Defense-associated sirtuin 2 (DSR2) systems are widely distributed across prokaryotic genomes, providing robust protection against phage infection. DSR2 recognizes phage tail tube proteins and induces abortive infection by depleting intracellular NAD+, a process that is counteracted by another phage-encoded protein, DSR Anti Defense 1 (DSAD1). Each DSR2 protomer consists of a conserved N-terminal Sirtuin (SIR2) domain, a C-terminal domain (CTD) and a middle domain (MD). DSR2 assembles into an elongated tetramer, with four NADase catalytic modules clustered in the center and the regulatory-sensing modules distributed at four distal corners.

To understand the structural basis of DSR2 anti-phage defense, we expressed the full-length Bacillus subtilis DSR2 protein in Escherichia coli BL21 and determined the cryo-EM structure at 4.15 Å. This structure is referred to as the apo DSR2 tetramer to distinguish it from the complex with the Tube protein (activator) and the DSAD1 (inhibitor) bound structures reported later. In this structure, four DSR2 subunits assemble into an autoinhibited homo-tetrameric assembly, forming a ~ 480 kDa bone-shaped supramolecular complex. Two DSR2 subunits first cross over to form an X-shaped dimer, mediated by the SIR2 and MD domains. The tetramer is then assembled by arranging two such dimers in a head-to-head orientation, facilitated by the SIR2 domain. The DSR2W143G/Y148G/Y552G/V556S/F559G/N563S mutant with disruption at the dimeric interface behaves as a monomer, whereas the DSR2I259S/Y260G mutant with disruption at the tetrameric interface behaves as a dimer. As expected, in the absence of activator binding, DSR2 showed no detectable in vitro NADase activity. The same arrangement and similar active sites of the SIR2 domains in the apo DSR2 tetramer and inactive ThsA suggest that the apo form of DSR2 represents the inactive conformation of the DSR2 complex. In contrast to the “loose” structure of the apo DSR2 tetramer (~256 Å in diameter), the DSR2H171A-Tube tetramer shows a more compact structure (~226 Å in diameter). Without phage infection, the apo DSR2 tetramer in cells adopts an inactive, loose conformation with its N-terminal SIR2 domain in a self-suppressed state.

>[2x]MVKVDLESKRYGEKLKEVFLMLDNNVVECIKEITESSRNGKLVFFVGAGVSTLSDYPQWWRLVDKYHEELYGSPKKGNYSSDEYLRIPQIFYNVKGEMAFDGILKDFFQVDKPTNPIHDKILAMNPAHVITTNYDNLIDTACWKRGKYFSVISAEEDVANATSSRYLLKVHGDFRKGFKGENVVLKEDDYLNYDQNYPLISNLMKTIIATHTIVFIGYGLGDYNINMLLNWVRKLQKDSFHKPFFIRTDPSPIENETLIYYENKGLRIIDAASLIDSNEYDYLERYSAVMDLLIESQENKFITKDDEVIDYIYGKISPLFALQYIRKIDLKHVFEYDYHFEVNGTVVRHKNKGFGYMERFFELKESCDERSKLSKKQYERFNALFNFFEKNGVICMAKDAGTLNTSIEINSLAYHGKYDVMKKFIEEQSVSIEDDYKKAFFLACLGRWEESYDLYSNIILNSIDESNGCVYYLSQINRYRIYQSITQAVTQFNGLGLLTFGRHYKPFTDEFLARIEREMTNFNIDDLFNGMPFEFQKKYKILEFLSDNQFLYDDTVKLFELTNKVRSEMSEGSYSFGMSSDIVVLLRLYDNLRFLYENCLWSVSFHEFHQYIRNSMSLLIEKAEYERTRDIDELGFSFFGKKSGFFMEYYDFVNISRHFKIDDIKNLERSCSIDKIRFGEQEKIEEYLVGIAEEITKQFSANGMNVVFYTQFISEAKAALYFAKYVKLSEEGLGKIVKALLFYFPERDLDIGKRYVWLERLTKCNELPKSIISIIDDFLVLQAEKHIDQNYSEVSSNGLYSRDYGALIKHFEKNFISKRLSEITLCLTQDKQKQIDFLFKLLPLLSTNAKSHLLSFKSVENINDLMNGIRIGLIDEFTPEHEELIIEYLETRKVNYIVEKEKGIQTFSSNDYMSTFGIWYFLEEINNSKMEEFIGMDDQYDFFVDPENFDYKKFIPSWLKNYNDKLLGKIAGNKHMKHHVIEVLKERVKNSNDKRYLEILMNYFI> MDGPGASAVVVRVGIPDLQQTKCLRLDPAAPVWAAKQRVLCALNHSLQDALNYGLFQPPSRGRAGKFLDEERLL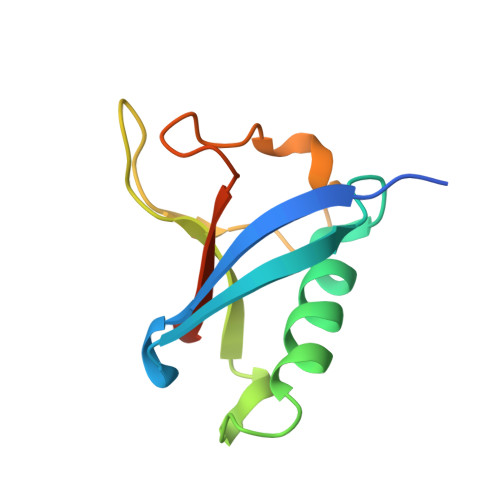QEYPPNLDTPLPYLEFRYKRRVYAQ>[6x]MGSSHHHHHHSQDPNSMETVLQIPYQKKTQIEKLLEFMYGLNEKEVQLIFRLLY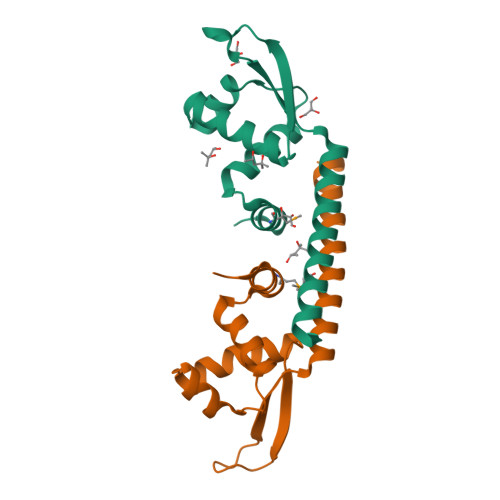SDTKLNIEELAEEFKVSKALISKSLSELANKGLIEREKVSNEGRKGRPIYVYYVDREQLFKRISRDLEELVQASIAKLKEYIFKS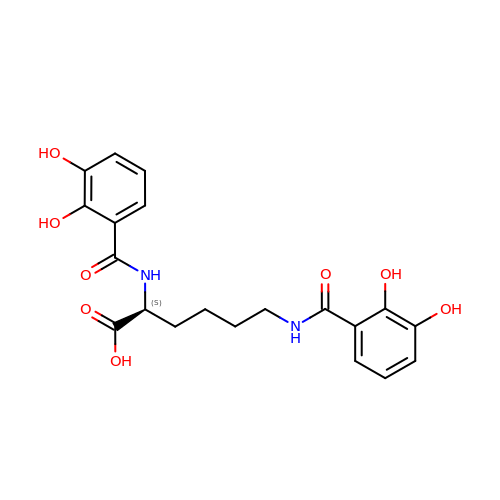Azotochelin | C20 H22 N2 O8 | KQPFLOCEYZIIRD-ZDUSSCGKSA-N>MASMTGGQQMGRGSMSTKAIYPGTFDPITNGHIDIITRAASMFDRVILAIAASPSKKPMFDLEERVALATTALQHLPNVEVMGFSDLMANFARAQQANILIRGLRAVADFEYEMQLAHMNRHLMPELESVFLM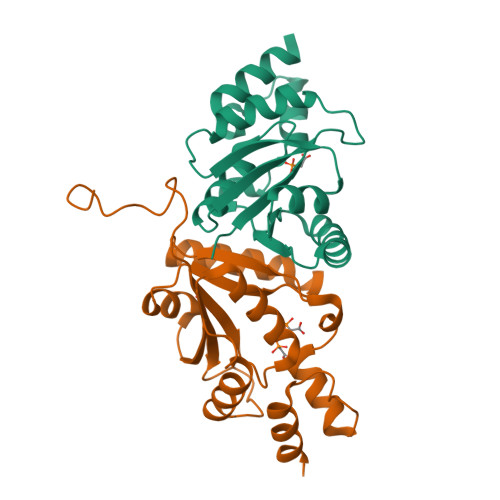PSKEWSFISSSLVKEVARHAGDVTHFLPANVHQALMEKLK[6x];> MASMTGG(2S)-2-amino-N-butyl-propanamide 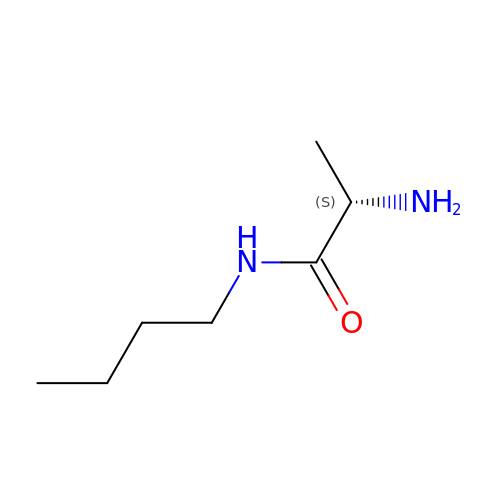| C7 H16 N2 O | XXYQJGUBGFEJMV-LURJTMIESA-N>GPHMAAAAMAAAAGGGAGAARSLSRFRGCLAGALLGDCVGSFYEAHDTVDLTSVLR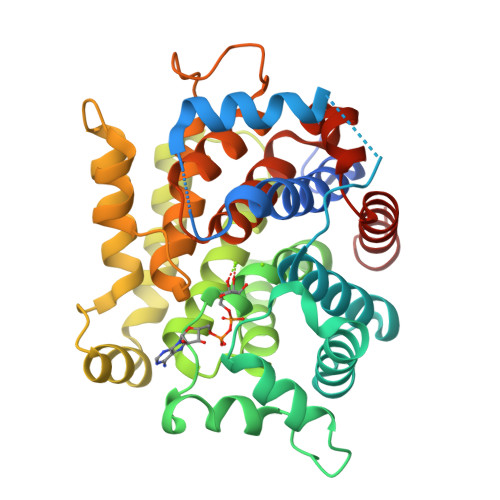HVQSLEPDPGTPGSERTEALYYTDDTAMARALVQSLLAKEAFDEVDMAHRFAQEYKKDPDRGYGAGVVTVFKKLLNPKCRDVFEPARAQFNGKGSYGNGGAMRVAGISLAYSSVQDVQKFARLSAQLTHASSLGYNGAILQALAVHLALQGESSSEHFLKQLLGHMEDLEGDAQSVLDARELGMEERPYSSRLKKIGELLDQASVTREEVVSELGNGIAAFESVPTAIYCFLRCMEPDPEIPSAFNSLQRTLIYSISLGGDTDTIATMAGAIAGAYYGMDQVPESWQQSCEGYEETDILAQSLHRVFQKS[4x]> MTMDFSDPDMEFLCLTRQKLMEATSIPFDGKKNCWVPDPDFGFVGAEIQSTKGDEVTVKTDKTQETRVVKKDDIGQRNPPKFEMNMDMANLTFLNEASILHNLRSRYESGFIYTYSGLFCIAINPYRRLPIYTQGLVDKYRGKRRAEMPPHLFSIADNAYQYMLQDRENQSMLITGESGAGKTENTKKVIQYFALVAASLAGKKDKKEEEKKKDEKKGTLEDQIVQCNPVLEAYGNAKTTRNNNSSRFGKFIRIHFGTQGKIAGADIETYLLEKSRVTYQQSAERNYHIFYQLLSPAFPENIEKILAVPDPGLYGFINQGTLTVDGIDDEEEMGLTDTAFDVLGFTDEEKLSMYKCTGCILHLGEMKWKQRGEQAEADGTAEAEKVAFLLGVNAGDLLKCLLKPKIKVGTEYVTQGRNKDQVTNSIAALAKSLYDRMFNWLVRRVNQTLDTKAKRQFFIGVLDIAGFEIFDFNSFEQLCINYTNERLQQFFNHHMFVLEQEEYKKEGIVWEFIDFGLDLQACIELIEKPMGILSILEEECMFPKASDTSFKNKLYDNHLGKNPMFGKPKPPKAGCAEAHFCLHHYAGSVSYSIAGWLDKNKDPINENVVELLQNSKEPIVKMLFTPPRILTPGGKKKKGKSAAFQTISSVHKESLNKLMKNLYSTHPHFVRCIIPNELKTPGLIDAALVLHQLRCNGVLEGIRICRKGFPNRIIYSEFKQRYSILAPNAVPSGFADGKVVTDKALSALQLDPNEYRLGNTKVFFKAGVLGMLEDMRDERLSKIISMFQAHIRGYLMRKAYKKLQDQRIG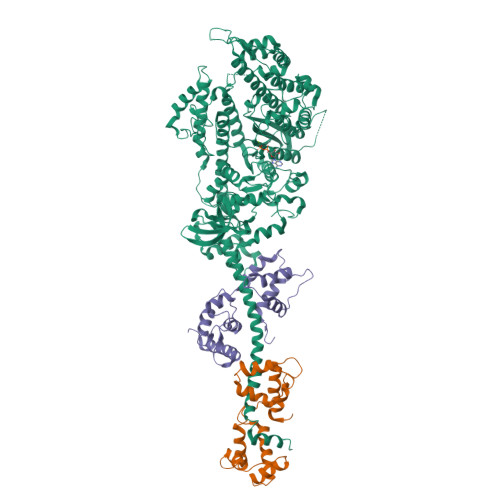LTLIQRNVRKWLVLRNWEWWRLFNKVKPLL;> AEEAPRRVKLSQRQMQELKEAFTMIDQDRDGFIGMEDLKDMFSSLGRVPPDDELNAMLKECPGQLNFTAFLTLFGEKVSGTDPEDALRNAFSMFDEDGQGFIPEDYLKDLLENMGDNFSKEEIKNVWKDAPLKNKQFNYNKMVDIKGKAEDED;> SQLTKDEIEEVREVFDLFDFWDGRDGDVDAAKVGDLLRCLGMNPTEAQVHQHGGTKKMGEKAYKLEEILPIYEEMSSKDTGTAADEFMEAFKTFDREGQGLISSAEIRNVLKMLGERITEDQCNDIFTFCDIREDIDGNIKYEDLMKKVMAGPFPDKSD> ASSTNLKDILADLIPKEQARIKTFRQQHGNTVVGQITVDMMYGGMRGMKGLVYETSVLDPDEGIRFRGYSIPECQKMLPKAKGGEEPLPEGLFWLLVTGQIPTEEQVSWLSKEWAKRAALPSHVVTMLDNFPTNLHPMSQLSAAITALN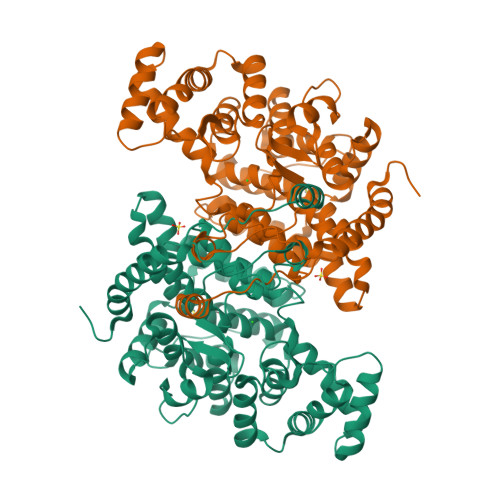SESNFARAYAEGIHRTKYWELIYEDCMDLIAKLPCVAAKIYRNLYREGSSIGAIDSKLDWSHNFTNMLGYTDAQFTELMRLYLTIHSDHEGGNVSAHTSHLVGSALSDPYLSFAAAMNGLAGPLHGLANQEVLVWLTQLQKEVGKDVSDEKLRDYIWNTLNSGRVVPGYGHAVLRKTDPRYTCQREFALKHLPHDPMFKLVAQLYKIVPNVLLEQGKAKNPWPNVDAHSGVLLQYYGMTEMNYYTVLFGVSRALGVLAQLIWSRALGFPLERPKSMSTDGLIKLVDSK>[3x]MQQLNPSEISALIKQRIGDLDTSATAKNEGTIVMVSDGIVRIHGLADAMYGEMIEFDGGLFGMALNLEQDSVGAVVLGNYLSLQEGQKARCTGRVLEVPVGPELLGRVVDALGNPIDGKGPIDAKLTDAVEKVAPGVIWRQSVDQPVQTGYKSVDTMIPVGRGQRELIIGDRQTGKTAMAIDAIIAQKNSGIKCVYVAIGQKQSTIANVVRKLEETGAMAYTTVVAAAAADPAAMQYLAPYSGCTMGEYFRDRGEDALIIYDDLSKQAVAYRQISLLLRRPPGREAYPGDVFYLHSRLLERASRVSAEYVEKFTNGAVTGKTGSLTALPIIETQAGDVSAFVPTNVISITDGQIFLETSLFNAGIRPAVNAGISVSRVGGSAQTKIIKKLSGGIRTALAQYRELAAFAQFASDLDEATRKQLEHGQRVTELMKQKQYAPYSIADQAVSVYASNEGYMADVEVKKIVDFDAALIAYFRSEYAPLMKQIDETGDYNKDIEAAIKAGIESFKATQTY;>MSSGRIIQIIGAVIDVEFERTSVPKIYDALQVDGTETTLEVQQQLGDGVVRTIAMGSTEGLKRGLTVTSTNAPISVPVGTATLGRIMDVLGRPIDEAGPVATEERLPIHRQAPSYAEQAASTDLLETGIKVIDLLCPFAKGGKVGLFGGAGVGKTVNMMELINNIAKAHSGLSVFAGVGERTREGNDFYHEMKDSNVLDKVAMVYGQMNEPPGNRLRVALTGLTMAEYFRDEKDENGKGRDVLLFVDNIYRYTLAGTEVSALLGRMPSAVGYQPTLAEEMGVLQERITSTKSGSITSIQAVYVPADDLTDPSPATTFAHLDATVVLSRDIASSGIYPAIDPLDSTSRQLDPLVVGQEHYEIARAVQNVLQRYKELKDIIAILGMDELAEEDKLVVYRARKIQRFFSQPFHVAEVFTGAPGKLVPLKETIRGFKGLLAGEYDHIPEQAFYMVGGIDEVIAKAEKL[3x];>[10x]MELTLGLVAIASAILIAFGALGTAIGFGLLGGRFLEAVARQPELAPQLQTRMFLIAGLLDAVPMIGVGIGLFFIFANPFVG;> MAAEEHALTSTEYIKHHLTNMTYGKMPDGTWKLAETAEEAHSMGFTAIHLDSMGWSIGLGVIFCLLFWIVARAANAGVPTKFQSAIEMIIEFVDSSVRDTFHGKSRLIAPLALTIFVWIFLMNLMDLIPVDWIPQVAAFVGANVFGMDPHHVYFKIVPSTDPNITLGMSLSVFVLILFYSIREKGVGGFVGELALNPFNPSNPVAKALLIPVNLILELVTFLARPISLALRLFGNMYAGELIFILIALLPFWIQWALSVPWAIFHILVITLQAFIFMMLTIVYLSMASEKH;>MNINLTLIGQAIA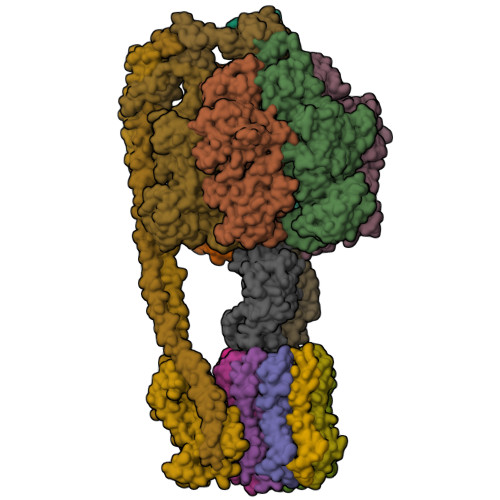FAFFVAFCMKFVWPPLINAISERQRKIADGLNAAEKAKADLADAQAQVKQELDAAKAQAAQLIEQANRRAAQLIEEARTQAAAEGERIRQQAKEAVDQEINSAREELRQQVAALAVTGAEKILNQQVDAEAHNAMLSQLAAKL[2x];> MAELLTLARPYAKAAFAYASEQGATDNWSNALQVLSAAVQDEAFSAYLNRPELTPAEQVKLFAKVLGEDQSQAVSNFLTLLADNDRLVLLPEIAAEYEQLKSQNNNNVDVVIESAFPLTAEQEQLLKSALEKRFNSTVTVSVEVKPELIAGVVIRAGDQVIDDSALNKLEKMRTRLLA;> MATMQCDVVSVKESIYSGAVTMLIAKGAGGELGILPGHAPLVTLLQPGPIRVLLENGTEEIVYVSGGVLEVQPHVVTVLADTAIRADNLDEAAILEARKNAEQLLANQKSDLDSAAALAALAETAAQLETIRKIKNRAQ;> MANLKEIRAKVASIKSTQKITRAMQMVAASKMRRAQERMAQGRPYADNMRRVIAHLVQANPEYKHRYMVDRPVKRVGYIIVSSDRGLAGGLNINLFKKVVQHVKAQQEQSIEVQFALIGQKAVSFFKNYGGKVLGATTQIGDAPSLEQLTGSVQVMLDAFDKGELDRIYLVSNGFVNAMTQKPKVEQLVPLAPAEEGDDLNRTYGWDYIYEPEAEELLNGLLVRYIESMVYQGVIENVACEQSARMVAMKAATDNAGQLIKDLQLIYNKLRQAAITQEISEIVGGAAAV>MKNKLKVLALTL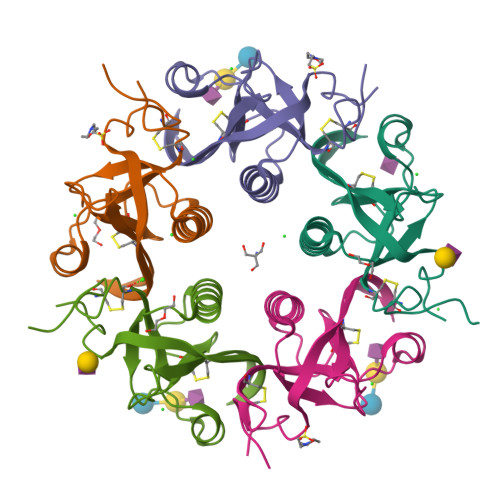ASLSSVCYANMADYNTYQSNVQINNLSYGVYRSGDKESQFFCVGLKRGSQVPNVHTICKIDVFGTHKQGFDNMLATARYYYATGEDVRIYYKENVWTDRNFTAAFSGNELIAITTCTSSDYCMGPTLPNLEHHHHHH[10x]Diphtheria toxin (DT) is secreted by Corynebacterium and causes disease in humans by inhibiting protein synthesis. DT consists of three domains—receptor (R-), translocation (T-), and catalytic (C-)—and similar to many other A-B toxins it enters the cell via the endosomal pathway. After the binding of the R-domain to the EGFR-like receptor on the cell surface, the toxin is endocytosed into the cell, and acidification inside the endosome promotes the requisite conformational change and membrane insertion of the T-domain followed by the translocation of the C-domain into the cytosol. Following translocation, the C-domain is proteolyzed from the R and T domains and proceeds to inhibit the EF2 translation factor, leading to the termination of protein synthesis and cell death.

DT was crystallized under varying buffer conditions in an effort to determine if conformational changes, particularly in the T-domain, are observed with a decreasing pH. Since the crystallization conditions were identical except for the buffer, the crystals of DT-5.0, DT-5.5, DT-6.0, and DT-7.0 have similar unit cell dimensions and diffraction resolutions. Overall, all of the structures are very similar, with RMSD deviations between the Cα atoms of 0.34 Å (997 residues, DT-5.5), 0.38 Å (999 residues, DT-6.0), and 0.41 Å (1000 residues, DT-7.0). One region that stands out is the TH2-TH3 region of the T-domain, which consistently displays large B-factors in each subunit of all structures. Interestingly, the residues between H223 to P234, which span TH2, appear to become more flexible at a lower pH. Analysis of the B-factors for each structure shows ordered TH2 residues in DT-7.0 and slightly higher B-factors in this region for DT-6.0 in each subunit (TH2-A and TH2-B). As such, these structures suggest that the structural stability of TH2 is pH-dependent. The set of the structures generated for mildly acidic pH values of 6, 5.5, and 5 retain essentially the same conformations, with the hotspots of partial unfolding highlighted by the elevated B-factors. We demonstrate that neither catalytic nor receptor-binding domains change their structure upon this acidification, while the T-domain undergoes a conformational change that results in the unfolding of TH2–3 helices.

>[2x]MGADDVVDSSKSFVMENFSSYHGTKPGYVDSIQKGIQKPKSGTQGNYDDDWEGFYSTDNKYDAAGYSVDNENPLSGKAGGVVKVTYPGLTKVLALKVDNAETIKKELGLSLTEPLMEQVGTEEFIKRFGDGASRVVLSLPFAEGSSSVKYINNWEQAKALSVELEINFETRGKRGQDAMYEYMAQACAGNRVRRSVGSSLSCINLDWDVIRDKTKTKIESLKEHGPIKNKMSESPNKTVSEEKAKQYLEEFHQTALEHPELSELKTVTGTNPVFAGANYAAWAVNVAQVIDSETADNLEKTTAALSILPGIGSVMGIADGAVHHNTEEIVAQSIALSSLMVAQAIPLVGELVDIGFAAYNFVESIINLFQVVHNSYNRPAYSPGHKTQPFLHDGYAVSWNTVEDSIIRTGFQGESGHDIKITAENTPLPIAGVLLPTIPGKLDVNKSKTHISVNGRKIRMRCRAIDGDVTFCRPKSPVYVGNGVHANLHVAFHRSSSEKIHSNEISSDSIGVLGYQKTVDHTKVNSKLSLFFEIKSMA2-ethoxy-8-(5-fluoranylpyridin-3-yl)-6-methyl-9-[[4-[[(1S,4S)-5-methyl-2,5-diazabicyclo[2.2.1]heptan-2-yl]methyl]phenyl]methyl]purine 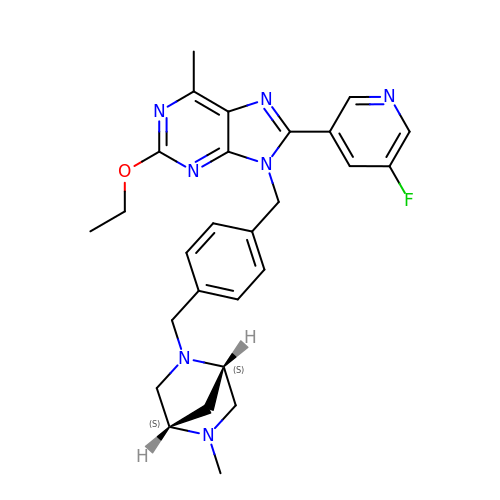| C27 H30 F N7 O | RIJUCCOLHSAZPO-GOTSBHOMSA-N> MRRAAMYEEGPPPSYESVVSAAPVAAALGSPFDAPLDPPFVPPRYLRPTGGRNSIRYSELAPLFDTTRVYLVDNKSTDVASLNYQNDHSNFLTTVIQNNDYSPGEASTQTINLDDRSHWGGDLKTILHTNMPNVNEFMFTNKFKARVMVSRLPTKDNQVELKYEWVEFTLPEGNYSETMTIDLMNNAIVEHYLKVGRQNGVLESDIGVKFDTRNFRLGFDPVTGLVMPGVYTNEAFHPDIILLPGCGVDFTHSRLSNLLGIRKRQPFQEGFRITYDDLEGGNIPALLDVDAYQASLKDDTEQGGGGAGGSNSSGSGAEENSNAAAAAMQPVEDMNDHAIRGDTFATRAEEKRAEAEAAAEAAAPAAQPEVEKPQKKPVIKPLTEDSKKRSYNLISNDSTFTQYRSWYLAYNYGDPQTGIRSWTLLCTPDVTCGSEQVYWSLPDMMQDPVTFRSTRQISNFPVVGAELLPVHSKSFYNDQAVYSQLIRQFTSLTHVFNRFPENQILARPPAPTITTVSENVPALTDHGT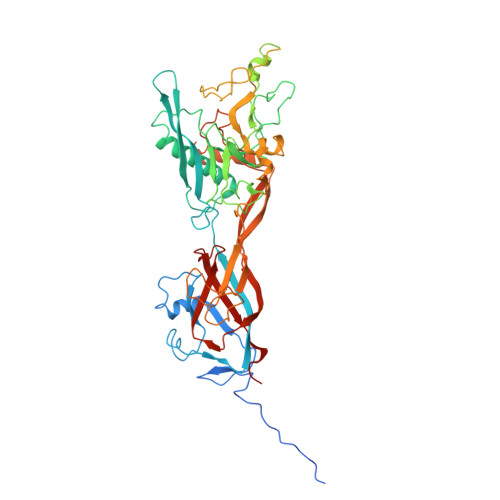LPLRNSIGGVQRVTITDARRRTCPYVYKALGIVSPRVLSSRTF>[2x]MPIQVLPPQLANQIAAGEVVERPASVVKELVENSLDAGATRIDIDIERGGAKLIRIRDNGCGIKKDELALALARHATSKIASLDDLEAIISLGFRGEALASISSVSRLTLTSRTAEQQEAWQAYAEGRDMNVTVKPAAHPVGTTLEVLDLFYNTPARRKFLRTEKTEFNHIDEIIRRIALARFDVTINLSHNGKIVRQYRAVPEGGQKERRLGAICGTAFLEQALAIEWQHGDLTLRGWVADPNHTTPALAEIQYCYVNGRMMRDRLINHAIRQACEDKLGADQQPAFVLYLEIDPHQVDVNVHPAKHEVRFHQSRLVHDFIYQGVLSVLQQQLETPLPLDDEPQPAPRSIPENRVAAGRNHFAEPAAREPVAPRYTPAPASGSRPAAPWPNAQPGYQKQQGEVYRQLLQTPAPMQKLKAPEPQEPALAANSQSFGRVLTIVHSDCALLERDGNISLLSLPVAERWLRQAQLTPGEAPVCAQPLLIPLRLKVSAEEKSALEKAQSALAELGIDFQSDAQHVTIRAVPLPLRQQNLQILIPELIGYLAKQSVFEPGNIAQWIARNLMSEHAQWSMAQAITLLADVERLCPQLVKTPPGGLLQSVDLHPAIKALKDE

DNA mismatch repair is essential for safeguarding the integrity of the genome. The repair process is executed by a series of proteins that together search, find and remove the mis-incorporated nucleotide from the newly synthesized strand. During this process, MutL plays an essential role by activating the UvrD helicase to remove a large section of the daughter strand containing the incorrectly incorporated nucleotide. Here we show that the Escherichia coli MutL protein binds to the 3′ end of the resected strand and blocks access of Pol I and Pol III.

In order to elucidate how MutL preferentially binds to 3′ resected DNA ends we determined the cryo-EM structure of MutL bound to 21 bp double stranded DNA substrate with a 21-nucleotide single stranded overhang in the presence of the non-hydrolysable ATP analogue AMPPNP to 3.7 Å resolution. Although we used full length MutL during sample preparation, in our structure we only see the N-terminal ATPase dimer and 13 bp of dsDNA plus 8 nucleotides of the single stranded overhang, resulting in a protein-DNA complex with a combined molecular weight of ∼85 kDa. Two N-terminal ATPase domains of MutL (MutLLN40) form the canonical dimer confirmation similar to the crystal structure of AMPPNP-bound MutLLN40 (37) with both monomers containing an AMPPNP molecule bound in the active site. The symmetry of the MutLLN40 dimer is broken by the DNA, with the double stranded section positioned on one end of the dimer, and the single stranded section on the opposite end. The single stranded overhang passes through a narrow cavity between the two MutL monomers and interacts with residues from both monomer A and B in a sequence independent manner. The specific recognition of the 3′ end of the dsDNA is performed by monomer B that thus positions the MutL dimer at the same DNA end that is the substrate for DNA polymerases. To do so, it interacts with the last base of the primer strand through a helix (residues 315–330) that positions R316 in the minor groove of the dsDNA. In addition, two histidines interact with the first unpaired nucleotide: H319 stacks onto the base, while H270 stacks onto the ribose of the same nucleotide. Positioning of a dsDNA substrate with a 5′ resected end results in a clash with monomer A, where K165 that normally protrudes into the major groove, now runs into one strand of the DNA (blue line).> GAHMKSTFKSEYPFEKRKAESERIADRFKNRIPVICEKAEKSDIPEIDKRKYLVPADLTVGQFVYVIRKRIMLPPEKAIFIFV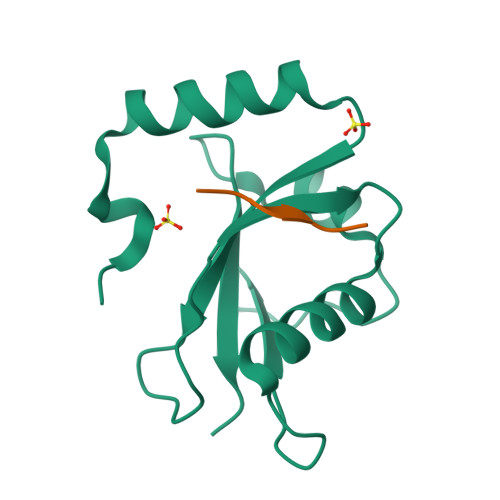NDTLPPTAALMSAIYQEHKDKDGFLYVTYSGENTFG;> SWQAIQ> MPFVNKQFNYKDPVNGVDIAYIKIPNAGQMQPVKAFKIHNKIWVIPERDTFTNPEEGDLNPPPEAKQVPVSYYDSTYLSTDNEKDNYLKGVTKLFERIYSTDLGRMLLTSIVRGIPFWGGSTIDTELKVIDTNCINVIQPDGSYRSEELNLVIIGPSADIIQFECKSFGHEVLNLTRNGYGSTQYIRFSPDFTFGFEESLEVDTNPLLGAGKFATDPAVTLAHELIHAGHRLYGIAINPNRVFKVNTNAYYEMSGLEVSFEELRTFGGHDAKFIDSLQENEFRLYYYNKFKDIASTLNKAKSIVGTTASLQYMKNVFKEKYLLSEDTSGKFSVDKLKFDKLYKMLTEIYTEDNFVKFFKVLNRKTYLNFDKAVFKINIVPKVNYTIYDGFNLRNTNLAANFNGQNTEINNMNFTKLKNFTGLFEFYKLLCVRGIITSKTKSLDKGYNKALNDLCIKVNNWDLFFSPSEDNFTNDLNKGEEITSDTNIEAAEENISLDLIQQYYLTFNFDNEPENISIENLSSDIIGQLELMPNIERFPNGKKYELDKYTMFHYLRAQEFEHGKSRIALTNSVNEALLNPSRVYTFFSSDYVKKVNKATEAAMFLGWVEQLVYDFTDETSEVSTTDKIADITIIIPYIGPALNIGNMLYKDDFVGALIFSGAVILLEFIPEIAIPVLGTFALVSYIANKVLTVQTIDNALSKRNEKWDEVYKYIVTNWLAKVNTQIDLIRKKMKEALENQAEATKAIINYQYNQYTEEEKNNINFNIDDLSSKLNESINKAMININKFLNQCSVSYLMNSMIPYGVKRLEDFDASLKDALLKYIYDNRGTLIGQVDRLKDKVNNTLSTDIPFQLSKYVDNQRLLSTFTEYIKNIINTSILNLRYESNHLIDLSRYASKINIGSKVNFDPIDKNQIQLFNLESSKIEVILKNAIVYNSMYENFSTSFWIRIPKYFNSISLNNEYTIINCMENNSGWKVSLNYGEIIWTLQDTQEIKQRVVFKYSQMINISDYINRWIFVTITNNRLNNSKIYINGRLIDQKPISNLGNIHASNNIMFKLDGCRDTHRYIWIKYFNLFDKELNEKEIKDLYDNQSNSGILKDFWGDYLQYDKPYYMLNLYDPNKYVD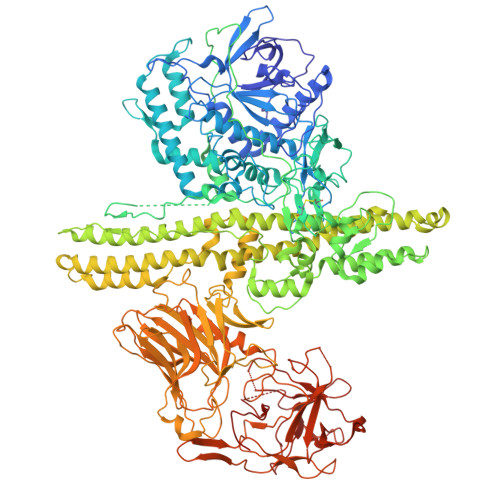VNNVGIRGYMYLKGPRGSVMTTNIYLNSSLYRGTKFIIKKYASGNKDNIVRNNDRVYINVVVKNKEYRLATNASQAGVEKILSALEIPDVGNLSQVVVMKSKNDQGITNKCKMNLQDNNGNDIGFIGFHQFNNIAKLVASNWYNRQIERSSRTLGCSWEFIPVDDGWGERPLLVPRGSHHHHHH> SMRKSREYEHVRRDLDPNEVWE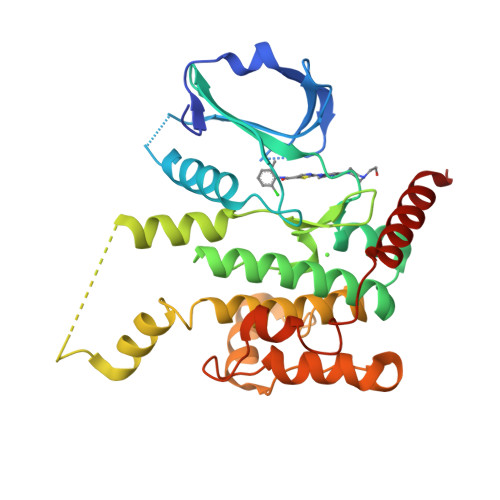IVGELGDGAFGKVYKAKNKETGALAAAKVIETKSEEELEDYIVEIEILATCDHPYIVKLLGAYYHDGKLWIMIEFCPGGAVDAIMLELDRGLTEPQIQVVCRQMLEALNFLHSKRIIHRDLKAGNVLMTLEGDIRLADFGVSAKNLKTLQKRDSFIGTPYWMAPEVVMCETMKDTPYDYKADIWSLGITLIEMAQIEPPHHELNPMRVLLKIAKSDPPTLLTPSKWSVEFRDFLKIALDKNPETRPSAAQLLEHPFVSSITSNKALRELVAEAKAEVMEE>MSVIAITGSASGIGAALKELLARAGHTVIGIDRGQADIEADLSTPGGRETAVAAVLDRCGGVLDGLVCCAGVGVTAANSGLVVAVNYFGVSALLDGLAEALSRGQQPAAVIV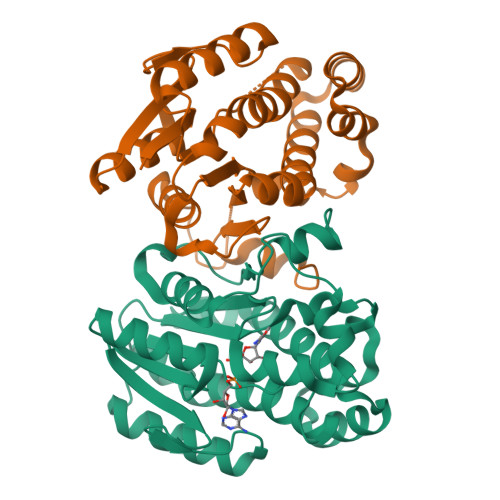GSIAATQPGAAELPMVEAMLAGDEARAIELAEQQGQTHLAYAGSKYAVTCLARRNVVDWAGRGVRLNVVAPGAVETPLLQASKADPRYGESTRRFVAPLGRGSEPREVAEAIAFLLGPQASFIHGSVLFVDGGMDALMRAKTF[2x]>[2x]GSKDYDELLKYYELHETIGTGGFAKVKLACHILTGEMVAIKIMDKNTLGSDLPRIKTEIEALKNLRHQHICQLYHVLETANKIFMVLEYCPGGELFDYIISQDRLSE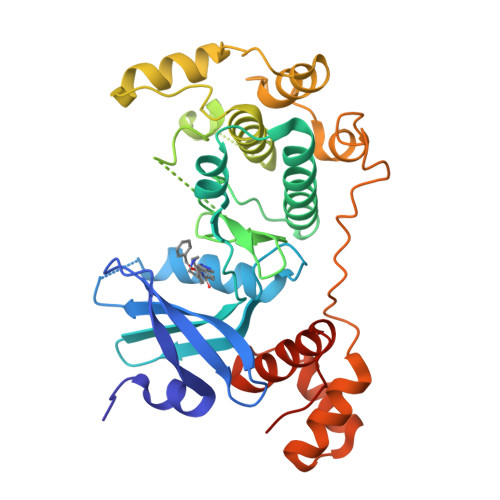EETRVVFRQIVSAVAYVHSQGYAHRDLKPENLLFDEYHKLKLIDFGLCAKPKGNKDYHLQTCCGSLAYAAPELIQGKSYLGSEADVWSMGILLYVLMCGFLPFDDDNVMALYKKIMRGKYDVPKWLSPSSILLLQQMLQVDPKKRISMKNLLNHPWIMQDYNYPVEWQSKNPFIHLDDDCVTELSVHHRNNRQTMEDLISLWQYDHLTATYLLLLAKKARGKPVRLRLSSFSCG> VEKLTADAELQRLKNERHEEAELERLK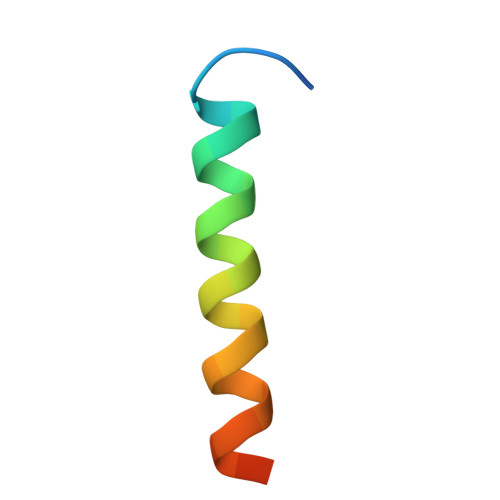SEY> MELSASATELLQDYMLTLRTKLS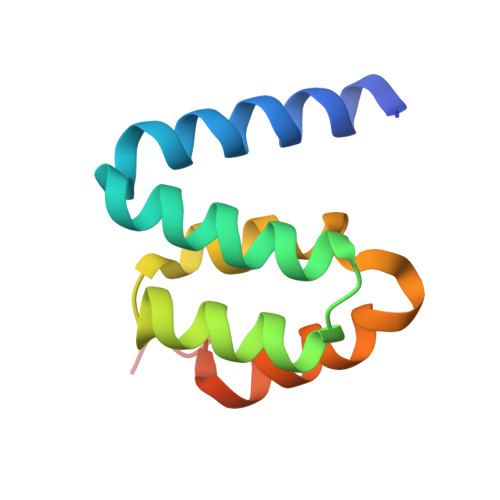SQEIQQFAALLHEYRNGASIHEFCINLRQLYGDSRKFLLLGLRPFIPEKDSQHFENFLETIGVKDLEHHHHHH>MTLSIPPSIQCQTEAACRLITRVTGDTLRAIHLYGSAVAGGLKPNSDIDLLVTICQPLTEAQRATLMQELLALSSPPGASAEKRALEVTVVLYSQLVPWCFPPSREMQFGEWLREDICQGIYEPAQQDWDMVLLITQILETSIPLKGERAERLFTPAPAAQLLKALRYPLDLWQSTADVQGDEYHIVLTLARIWYTLSTGRFTSKDAAADWLLPQLPEDYAATLRAAQREYLGLEQQDWHILLPAVVRFVDFAKAHIPTQFTKGHHHHHH[2x]

Aminoglycoside (3″)(9) adenylyltransferase AadA from Salmonella enterica belongs to the ANT(3″)-Ia family and catalyzes the magnesium-dependent O-adenylation of streptomycin and spectinomycin at positions 3″ and 9, respectively. Modification of streptomycin and spectinomycin by O-phosphorylation or O-nucleotidylation prevents the drugs from binding to their respective binding sites on the ribosome (for reviews, see Refs. 9 and 10). In the apo state, AadA has a monomeric two-domain structure with the active site located between an N-terminal adenylyltransferase domain and a C-terminal helical domain. We here present crystal structures of wild type (WT) AadA with ATP or ATP and streptomycin and of an active-site mutant in complex with ATP and streptomycin or dihydrostreptomycin.

Cocrystallization of WT AadA with ATP and magnesium yielded well-diffracting crystals. The crystals grew in a new space group, P32, with two molecules in the asymmetric unit, and the complete atomic structure could be built and refined to 1.9-Å resolution. The two molecules of AadA display close-to-identical structures (root mean square deviation (r.m.s.d.) of 0.1 Å over 261 Cα atoms). This structure represents a native state of the enzyme prior to binding of aminoglycoside substrate. To accommodate binding of ATP and magnesium, compared with the apo structure, the main part of the C-terminal domain rotates 11° relative to the N-terminal domain around the first helix of the C-terminal domain (helix 7), resulting in a shift of up to 4 Å. There are also local conformational changes of the 202–206 loop region directly linked to the interaction with ATP. The structure shows clear electron density for ATP and two magnesium ions in the interdomain cleft. In the N-terminal domain, Asp-47, Asp-49, and Glu-87 together with the phosphates of ATP coordinate the two magnesium ions. In addition, the phosphates make interactions with Ser-36 and Ser-46 in the N-terminal domain and Arg-192, Lys-205, and Tyr-231 in the C-terminal domain. The ribose is in C2′ endo conformation with both hydroxyl groups involved in hydrogen bonding to Asp-130. The adenine base is in syn conformation, packing between Leu-133, Leu-166, Thr-189, Arg-192, Ile-193, and Phe-202, and makes a single hydrogen bond to Thr-196 of the protein.> LPDSVDWREKGCVTEVKYQGS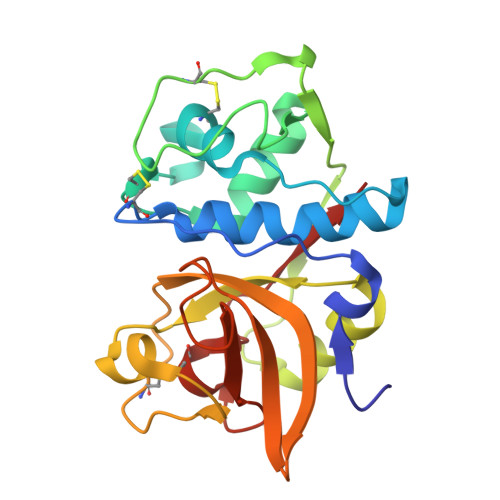CGASWAFSAVGALEAQLKLKTGKLVSLSAQNLVDCSTEKYGNKGCNGGFMTTAFQYIIDNKGIDSDASYPYKAMDLKCQYDSKYRAATCSKYTELPYGREDVLKEAVANKGPVSVGVDARHPSFFLYRSGVYYEPSCTQNVNHGVLVVGYGDLNGKEYWLVKNSWGHNFGEEGYIRMARNKGNHCGIASFPSYPEI S-Dihydrowogonin | C16 H14 O5 | 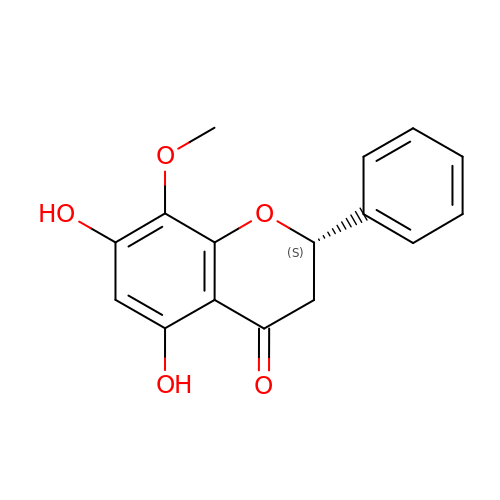FKAOWOSRYSMEBS-ZDUSSCGKSA-N1-(2-NITROPHENYL)ETHYL UDP-GALACTOSE | C22 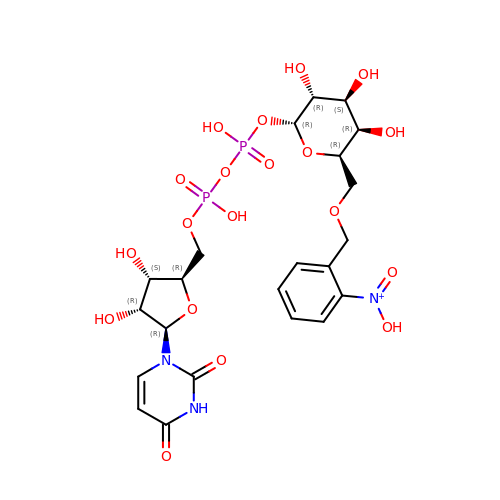H30 N3 O19 P2 | NGBDXGVIYRIOPC-DZEIOYJHSA-N> ASWSHPQFEKGASGAAESKPTPQSTFTGPIVVDPITRIEGHLRIMVEVENGKVKDAWSSSQLFRGLEIILKGRDPRDAQHFTQRACGCCTYVHALASSRCVDDAVKVSIPANARMMRNLVMASQYLHDHLVHFYHLHALDWVDVTAALKADPNKAAKLAASIAPARPGNSAKALKAVQDKLKAFVESGQLGIFTNAYFLGGHKAYYLPPEVDLIATAHYLEALHMQVKAASAMAILGGKNPHTQFTVVGGCSNYQGLTKDPLANYLALSKEVCQFVNECYIPDLLAVAGFYKDWGGIGGTSNYLAFGEFATDDSSPEKHLATSQFPSGVITGRDLGKVDNVDLGAIYEDVKYSWYAPGGDGKHPYDGVTDPKYTKLDDKD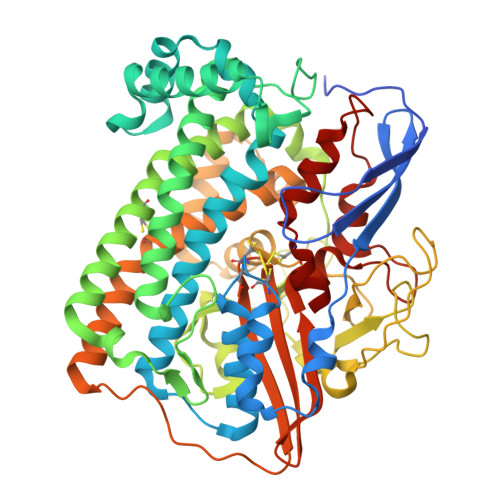HYSWMKAPRYKGKAMEVGPLARTFIAYAKGQPDFKKVVDMVLGKLSVPATALHSTLGRTAARGIETAIVCANMEKWIKEMADSGAKDNTLCAKWEMPEESKGVGLADAPRGALSHWIRIKGKKIDNFQLVVPSTWNLGPRGAQGDKSPVEEALIGTPIADPKRPVEILRTVHAFDPCIACGVH> GDQEPPLYVNENDIFTSPTRIEATLNGLYAAIKNTGTKSLMGGKSYLVFDNRGDDVINISNNLVTLFNTYNMNVGITDAENADTWTYAYLAINKVNTFLQSLEGAREVAGENYDRYVQEAKFVRALAYYYLNNLYPTPYSVNPDAKSVPLRLTAEAGTENNNMPRSTVKQIYEHILSDLENISALDTEVNTYTGVTHATQAAANMLKMRVYMAMNEWDKAITAGELVTGYSLPEDVTLIYKAPYFSQESIFSLPMADTNIPNTQQSLAEYYYDGKIMLIDTKSGIMSKPDYSLATDKRIIAFKGEKDLLMKFTDAKTKLQWVPIFRYAETLLDLAECYANKAGGEATAKSLLKQVRGRS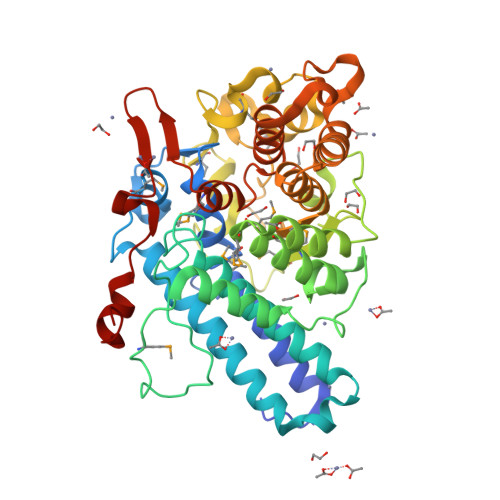VDAATDPLNIDNLSGDALKEAIYNEKRLEFIGEGIRGIDIMRRGEHFIKVGENETINVGPSDEKYTWPIPQVELLLNKDINK> MYRYEKKGPKRGVALYSYSAEFGLTKTLEDCFEDLHDMGAHGIEILANTHIENYPYPTDEWVEKWWRLCDKYEIVP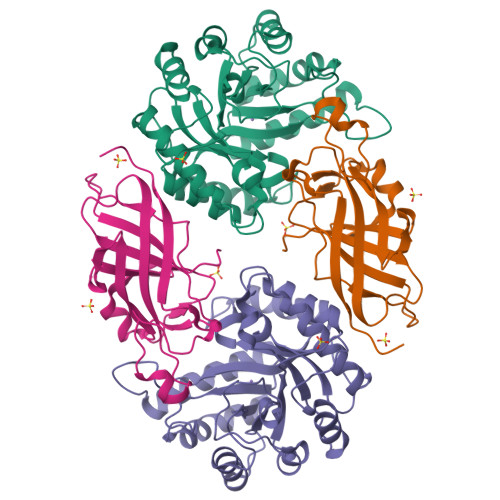VEYGNWIDSHVLGDRDLTTEESVEMLKRDIRLAHRLGFTVMRTKMPVINDLLEPVENWKEIIKGALPLAEELGIKMCPEIHTPSNLKGKLVNDFVEFIKETGTKNFGLNIDFSVFRTSFAEGEWVDPNYTPNKPEDIIPLLPYVYCCHAKFIHMSDDFKETTIPYEEVVKTMEDNGYEGYLLSEYEGADKYDEGYEVGQTLRKHHILLKNLLGD;> MEKQVIQSVGFRNIKNGNGEITGFQFKVKLPYYRGVFLSQIRPGTLFVDGQKIEKDQITWTINGEEYTNQEMRGDFKTHWATTKPAVLKVKMPGGLAQGYHDLKYGFCFTSSYMPPIIQDGLDPDKESMVYMPEFGHHVNERRLLIVKLAAALEHHHHHH>GENIVCRVICTTGQIP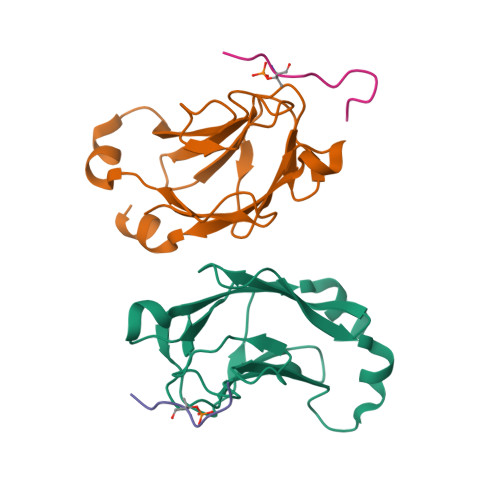IRDLSADISQVLKEKRSIKKVWTFGRNPACDYHLGNISRLSNKHFQILLGEDGNLLLNDISTNGTWLNGQKVEKNSNQLLSQGDEITVGVGVESDILSLVIFINDKFKQCL[2x];>[2x]SLEVTEADATFAK> MEKFVLSLDEGTTSARAIIFDRESNIHGIGQYEFPQHYPRPGWVEHNPEEIWDAQLRAIKDAIQSARIEPNQIAAIGVTNQRETTLVWDKDGKPLYNAIVWQCRRTAEMVEEIKREYGTMIK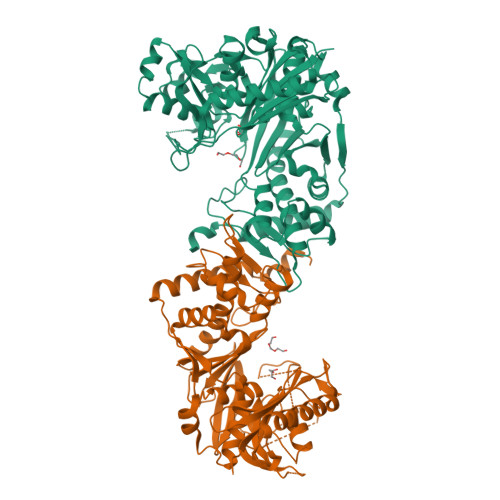EKTGLVPDAYFSASKLKWLLDNLPGLREKAEKGEVMFGTVDTFLIYRLTGEHVTDYSNASRTMLFNIKKLDWDDELLELFDIPESVLPEVRESSEVYGYTKKELLGAEIPVSGDAGDQQAALFGEAAFEAGMVKATYGTGSFILVNTDEMVLYSDNLLTTIAWGLNGRVSYALEGSIFVTGAAVQWLRDGIKIIKHASETEELATKLESNEGVYFVPAFVGLGAPYWDQFARGIIIGITRGTGREHLARATLEAIAYLTRDVVDEMEKLVQIKELRVDGGATANDFLMQFQADILNRKVIRPVVKETTALGAAYLAGLAVDYWADTREIAELWKAERIFEPKMDEKTRERLYKGWKEAVKRAMGWAKVVDSAKSN;>[3x]MEKFVLSLDEGTTSARAIIFDRESNIHGIGQYEFPQHYPRPGWVEHNPEEIWDAQLRAIKDAIQSARIEPNQIAAIGVTNQRETTLVWDKDGKPLYNAIVWQCRRTAEMVEEIKREYGTMIKEKTGLVPDAYFSASKLKWLLDNVPGLREKAEKGEVMFGTVDTFLIYRLTGEHVTDYSNASRTMLFNIKKLDWDDELLELFDIPESVLPEVRESSEVYGYTKKELLGAEIPVSGDAGDQQAALFGQAAFEAGMVKATYGTGSFILVNTDEMVLYSDNLLTTIAWGLNGRVSYALEGSIFVTGAAVQWLRDGIKIIKHASETEELATKLESNEGVYFVPAFVGLGAPYWDQFARGIIIGITRGTGREHLARATLEAIAYLTRDVVDEMEKLVQIKELRVDGGATANDFLMQFQADILNRKVIRPVVKETTALGAAYLAGLAVDYWADTREIAELWKAERIFEPKMDEKTRERLYKGWKEAVKRAMGWAKVVDSAKSN>[2x]MERTFVMIKPDGVQRGLIGEIISRFERKGLKIVAMKMMRISREMAEKHYAEHREKPFFSALVDYITSGPVV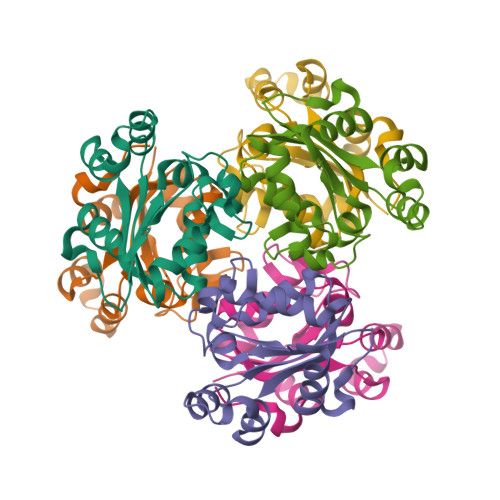AMVLEGKNAVEVVRKMVGATNPKEAAPGTIRGDFGLDVGKNVIHASDSPESAEREISLFFKDEELVEW>MVFSKVAVAASALSLGAYAIDAQINVDLQARYQSVDGFGCSQAFQRAEDIFGKYGLSPKNQSYVLDLMYSEERGAGFTILRNGIGSSNSSTSNLMNSIEPFSPGSPSSTPNYTWDHYNSGQFPLSQQARARGLPYIYADAWSAPGYMKTNQDENWSGFLCGIEGETCPSGDWRQAYADYLVQYVKFYAESGVPVTHLGFLNEPQEVVSYASMGSNGTQAAEFVKILGQTLEREGIDIELTCCDGVGWSEQEAMIPGLQVVGPDGKSAEDYLSVVTGHGYSSAPTFPLSTKRRTWLTEWTDLSGAFTPYTFFADGGAGEGMTWANHIQTAFVNANVSAFIYWIGAENSTTNSGMINLINDEV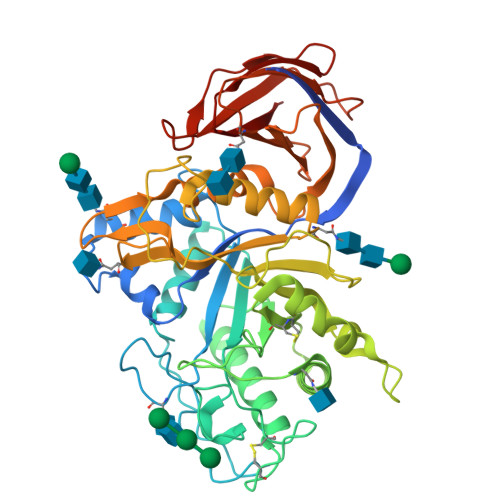IPSKRFWSMASFSKFVRPNAQRVKATSSDASVTVSAFENTNGVVAIQVINNGTSAASLTIDLGKTHKEVKKVVPWVTSNDYDLEEMSEIDVKHNSFLASVPARSLTSFVTECE[2x]Cut-and-paste DNA transposition requires a transposase, often encoded within the transposon, which binds sequence-specifically to the transposon IRs, makes a staggered double-strand break at each IR, and then inserts the cleaved transposon ends (together with the gene they encompass) at a new genomic location. mariner/Tc1 transposons usually integrate at TA dinucleotides, resulting in signature duplication of this sequence either side of the transposon. The well characterized mariner transposon Mos1, found in Drosophila mauritiana, has 28-bp inverted repeats that differ by 4 bp. The inner part of the IRR DNA sequence is recognized by the Mos1 DNA-binding domain of one transposase monomer, in cis; this domain (residues 1–112) comprises two helix-turn-helix (HTH) motifs connected by a minor groove-binding linker. The outer IRR sequence (containing three unpaired bases at the reactive 3′ end that mimic the product of the staggered double-strand break) is recognized by the catalytic domain of the other transposase monomer, in a trans arrangement.

Crystals of the Mos1 IRL PEC were formed by mixing full-length Mos1 transposase (T216A mutant) with duplex IRL DNA. This had a 3-nt overhang at the 3′ end of the transferred strand, mimicking the product of staggered transposon excision. The Mos1 IRL PEC structure has a similar overall architecture to the Mos1 IRR PEC described previously and comprises a transposase dimer bound to two IRL DNA molecules in a crossed configuration; one IRL DNA is bound by the DNA-binding domain of one monomer and the catalytic domain of the other monomer, and vice versa. As before, two additional IRL DNA duplexes interact with the catalytic domains, possibly occupying the binding sites of target DNA. In the Mos1 IRL PEC, the linker is displaced out of the minor groove, by a maximum of 1.7 Å at the amide bond between His-65 and Gly-66, as compared with its position in the IRR PEC. This is due in part to the higher GC content of the IRL sequence in this region as compared with the IRR sequence; the guanine 2-amino group adds bulk and hydrogen bond donors in the minor groove that obstruct transposase linker binding. Moreover, the pyrimidine-specific interaction between T16 O2 and the backbone amide of Lys-67 in the IRR PEC is lost in the IRL PEC because T16 is replaced by G in the IRL sequence. Additionally, the O2 of C41 (base-paired with G16) repels the backbone carbonyl of Lys-67 in the PEC IRL structure. Surprisingly, in the IRL PEC structure, there are additional interactions between the N1H and NH2 of G56 and the side-chain carboxylates of Glu-345, the C-terminal transposase residue.

>[2x]MSSFVPNKEQTRTVLIFCFHLKKTAAESHRMLVEAFGEQVPTVKTCERWFQRFKSGDFDVDDKEHGKPPKRYEDAELQALLDEDDAQTQKQLAEQLEVSQQAVSNRLREMGKIQKVGRWVPHELNERQMERRKNTCEILLSRYKRKSFLHRIVTGDEKWIFFVNPKRKKSYVDPGQPATSTARPNRFGKKTMLCVWWDQSGVIYYELLKPGETVNAARYQQQLINLNRALQRKRPEYQKRQHRVIFLHDNAPSHTARAVRDTLETLNWEVLPHAAYSPDLAPSDYHLFASMGHALAEQRFDSYESVKKWLDEWFAAKDDEFYWRGIHKLPERWEKCVASDGKYFE> MAKVYKDLREFLEVLEQEGQLIRVKEEVNPEPDIAAAGRAAANLGKNQPAVFFEKIKGYKYSVVTNVHGSWQNHALMLGLDKNTSTKDQFYELNRRWDKFPVPPNVVKREAAPCKENVIDKDINLFEILPLYRINEQDGGFYISKASVVTADPEYPDDFNKLNVGTYRIQVKDRDRVGIQALAMHDIAVQLEKAEAENKPLPIAITIGNNPLVTFMASTPVGYNQNEYEFVGALQDGVPMDIVKSDLYDHLYVPAGSEVVLEGHIIPRVRTVEGPFGEFPGSYSGA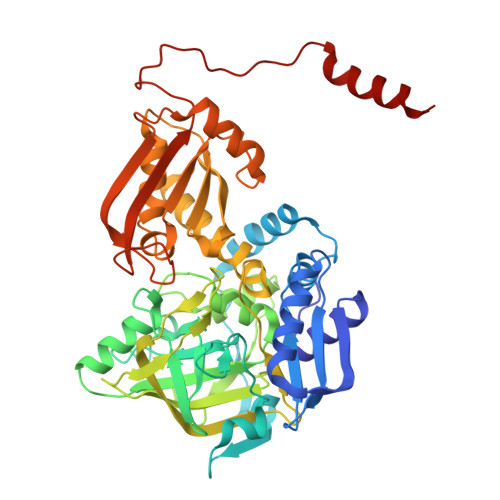RLQCEVKIDRITHRTNPIFENLYLGIPWTEIDYLMALNTSVPLYKQLKETMPEVVAVNAMYTHGIGVIISTKVRYGGYAKGVAFRLLSTPHGMPYSKIVIVVDEFVDPFNLEQVMWALTTRVHPGKDVSIIENCPGMPLDPSTNPPGMHTKMIIDATTPVPPEPNPRETQLLDPPDGTEEWEEKLKELLKNQNR> QRRLYDQAKAALAKGNSAPYMASRSALRDYPLEPYLAYDELTHRLKSASNEEVERFLTEHGDLPQIGWLKLRWLRLLADRGDWKTFVNYYDPKLNFTELDCLYGQYQLGHGQKAEGYATSERLWLVGKSQPAACDTLFGLWQGEGQLTEEKVWKRLKLAAEARNYSLASHLAQRLPTLGNQGALMVSVAQNPAQLSQTGRFSQRDHATADVVGLGLRRLARQDPEKALSLLDYYSSALPFSSDEKVAIAREIGLSLAKRFDPRALPLMTQYDPGLRDNTVTEWRTRLLLRLGRWDEAYALTRKLPQDLAATSRWRYWQARSLQLAQPNSKEPIALYQKLAGERDFYGFLAADRLSVPYKLGNRPAHIDPRVLQRVRNAASTRRAMEFFNRGEVINARREWYHAARLFDRDELIAQARLAYDMQWYFPAIRSISQAQYWDDLDIRFPMAHRATLVREAKNRGLH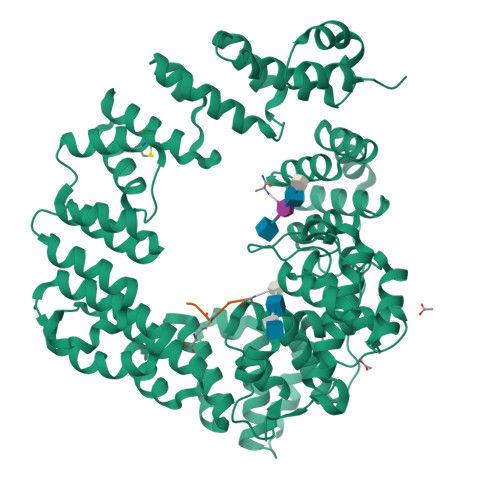SSWIFAITRQQSAFMSDARSGVGATGLMQLMPGTAKETSRKFGIPLASTQQLIVPDVNIRLGAAYLSQVHSQFNGNRVLASAAYNAGPGRVRQWLKDTRHLAFDVWIETIPFDETRQYVQNVLSYAVIYGQKLNAPQPIVDWHERYFDDF;> AEKAA> SGVFEVHNNCPYTVWAAATPVGGGRRLERGQSWWFWAPPGTKMARIWGRTNCNFDGAGRGWCQTGDCGGVLECKGWGKPPNTLAEYALNQFSNLDFWDISVIDGFNIPMSFGPTKPGPGKCHGIQCTANINGECPGSLRVPGGCNNPCTTFGGQQYCCTQGPCGPTELSRWFKQRCPDAYSYPQ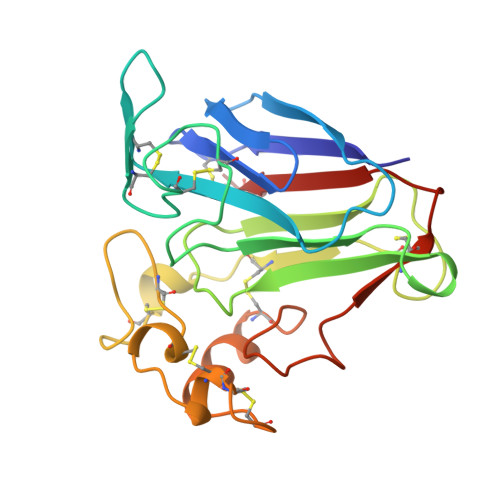DDPTSTFTCTSWTTDYKVMFCPYG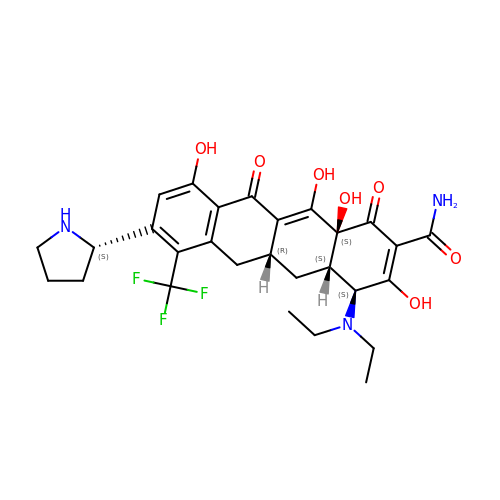(4S,4aS,5aR,12aS)-4-(diethylamino)-3,10,12,12a-tetrahydroxy-1,11-dioxo-8-[(2S)-pyrrolidin-2-yl]-7-(trifluoromethyl)-1,4,4a,5,5a,6,11,12a-octahydrotetracene-2-carboxamide | C28 H32 F3 N3 O7 | IDWTZCZXXFOLNV-DOYYSQEVSA-N> GSDWVIPPINLPENSRGPFPQELVRIRSG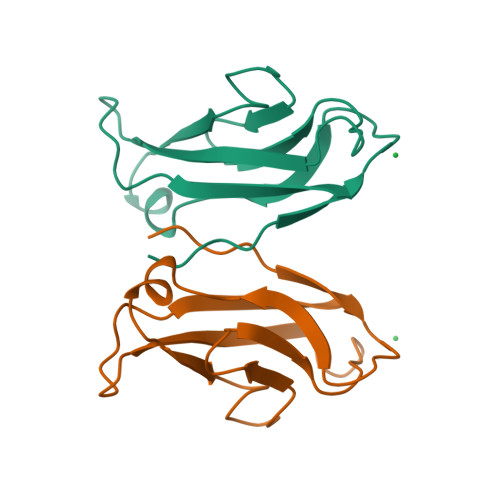RDKNLSLRYSVTGPGADQPPTGIFIINPISGQLSVTKPLDRELIARFHLRAHAVDINGNQVENPIDIVINVIDMNDNRPEF>[2x]MVKL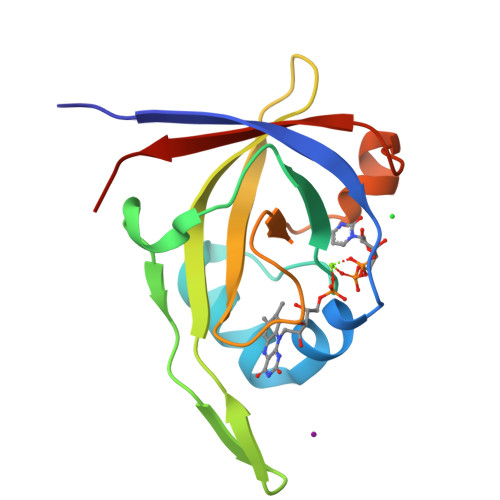MIIEGEVVSGLGEGRYFLSLPPYKEIFKKILGFEPYEGTLNLKLDREFDINKFKYIETEDFEFNGKRFFGVKVLPIKILIGNKKIDGAIVVPKKTYHSSEIIEIIAPMKLREQFNLKDGDVIKILIKGDKDE>[2x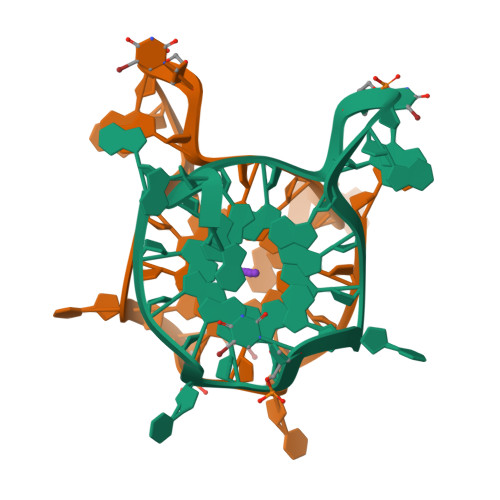]AGGGCGGUGTGGGAAUAGGGAA>[2x]GPKVPESGSMNLAAAERKKTGDLSVRSLHDIVKPEDFVLNSEHLTTVLVAVPKSLKSDFEKSYETLSKNVVPASASVIAEDAEYVLFNVHLFKKNVQEFTTAAREKKFIPREFNYSEELIDQLKKEHDSA;>MSSAITALTPNQVNDELNKMQAFIRKEAEEKAKEIQLKADQEYEIEKTNIVRNETNN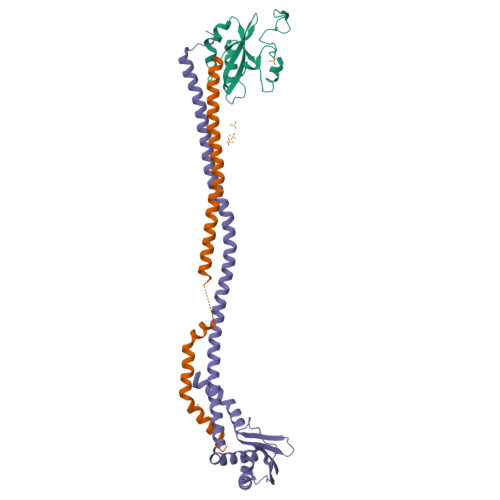IDGNFKSKLKKAMLSQQITKSTIANKMRLKVLSAREQSLDGIFEETKEKLSGIANNRDEYKPILQSLIVEALLKLLEPKAIVKALERDVDLIESMKDDIMREYGEKAQRAPLEEIVISNDYLNKDLVSGGVVVSNASDKIEINNTLEERLKLLSEEALPAIRLELYGPSKTRKFFD[2x];>GPKVPMSQKNGIATLLQAEKEAHEIVSKARKYRQDKLKQAKTDAAKEIDSYKIQKDKELKEFEQKNAGGVGELEKKAEAGVQGELAEIKKIAEKKKDDVVKILIETVIKPSAEVHINAL[2x]Poxvirus encoded M2 protein is a member of the poxvirus immune evasion family and plays roles in host immunomodulation via the regulation of innate immune response mediated by the NF-κB pathway and adaptive immune response mediated by B7 ligands. Here we reveal that MPXV M2, co-existing as a hexamer and a heptamer, recognizes human B7.1 and B7.2 (hB7.1/2) with high avidities. The binding of oligomeric MPXV M2 interrupts the interactions of hB7.1/2 with CD28 and CTLA4 and subverts T cell activation mediated by B7.1/2 costimulatory signals. Cryo-EM structures of M2 in complex with hB7.1/2 show that M2 binds to the shallow concave face of hB7.1/2 and displays sterically competition with CD28 and CTLA4 for the binding to hB7.1/2.

We finally determined three complex structures, M2-hB7.1 hexamer, M2-hB7.2 hexamer, and M2-hB7.2 heptamer, at an overall resolution of 3.04, 2.7, and 3.12 Å, respectively. We could not obtain a three-dimensional reconstruction of the M2-hB7.1 heptamer complex, partially due to the few cryo-EM particles of this complex on the cryo-EM grids. The resulting structures reveal that M2 forms an oligomeric ring structure with B7 proteins binding to the outer face of the M2 ring in a 1:1 stoichiometry. Structural analysis reveals that M2 interacts with hB7.1 and hB7.2 similarly. The interfaces of the two complex structures have very similar atomic contacts and bury a total accessible surface area of 1760 and 1617 Å2, respectively. M2 binds to hB7.1/2 side-by-side via β-strand complementation mediated by the C-terminal half of the M2 β11 and the N-terminal part of the hB7.1/2 G strand. The long C-terminal loop of M2 sits on top of the shallow concave surface, formed by the natural twist of strands G, F, C, and C’ of hB7.1/2. Extensive residues from the C-terminal loop, β8-β9 loop, and β10-β11 loop, and to a lesser extent, the β8, β9, β10, and β11 strands form a network of both van der Waals and hydrogen bonding interactions with residues from strands G, F, C, and C’ of hB7.1/2. Specifically, residues E122, K123, F126, K127, R128, and E133 from hB7.1, and residues M120, R122, Q125 as well as N127 from hB7.2 form hydrogen bonds with corresponding residues of M2 protein. There is a total of 12 residues on GFCC’ strands as well as CC’- and FG-loops of hB7.1 reside in the CTLA4-hB7.1 interface; however, 8 of them are also contacted by M2.

>VEYKNTICPPRQDYRYWYFVAELTIGVNYDINSTIIGECHMSESYIDRNANIVLTGYGLKINMTIMDTDQRFVAAAEGVGKDNKLSVLLFTTQRLDKVHHNISVTITCMEMNCGTTKYNSDLPESIHKSSSCDITINGSCVTCVNLETDPTKINPHYLHPKNKYLYHNSEYSMRGSYGVTFIDELNQCLLDIKELSYDICYRE[6x];>VIHVTKEVKEVATLSCGHNVSVEELAQTRIYWQKEKKMVLTMMSGDMNIWPEYKNRTIFDITNNLSIVILALRPSDEGTYECVVLKYEKDAFKREHLAEVTLSVKADFPTPSISDFEIPTSNIRRIICSTSGGFPEPHLSWLENGEELNAINTTVSQDPETELYAVSSKLDFNMTTNHSFMCLIKYGHLRVNQTFNWNTT[6x]> MRVLILGVNGFIGNHLTERLLREDHYEVYGLDIGSDAISRFLNHPHFHFVEGDISIHSEWIEYHVKKCDVVLPLVAIATPIEYTRNPLRVFELDFEENLRIIRYCVKYRKRIIFPSTSEVYGMCSDKYFDEDHSNLIVGPVNKPRWIYSVSKQLLDRVIWAYGEKEGLQFTLFRPFNWMGPRLDNLNAARIGSSRAITQLILNLVEGSPIKLIDGGKQKRCFTDIRDGIEALYRIIENAGNRCDGEIINIGNPENEASIEELGEMLLASFEKHPLRHHFPPFAGFRVVESSSYYGKGYQDVEHRKPSIRNAHRCLDWEPKIDMQETIDETLDF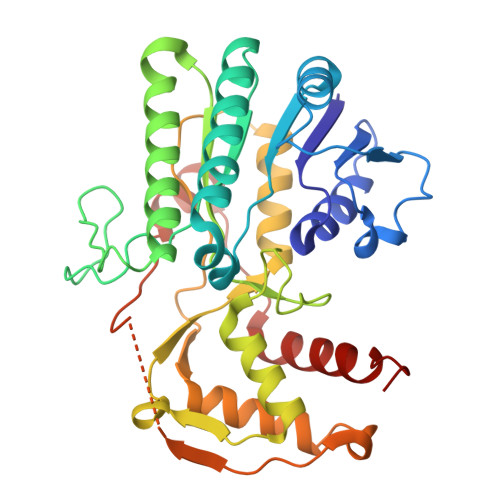FLRTVDLTD>EPELLFILVA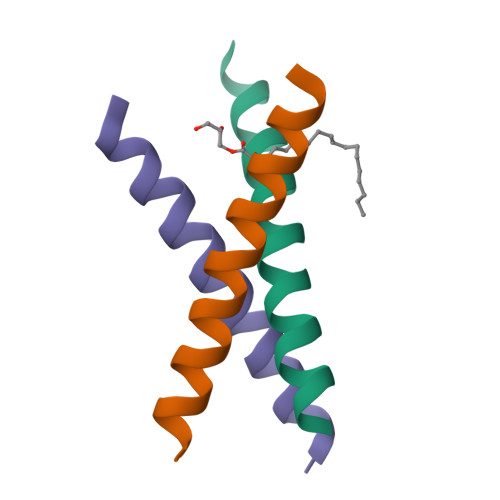ILGGLFGAIVAFLLALRRLC[4x]> IVGGTASVRGEWPWQVTLHTTSPTQRHLCGGSIIGNQWILTAAHCFYGVESPKILRVYSGILNQSEIKEDTSFFGVQEIIIHDQYKMAESGYDIALLKLETTVGYGDSQRPICLPSKGDRNVIYTDCWVTGWGYRKLRDKIQNTLQKAKIPLVTNEECQKRYRGHKITHKMICA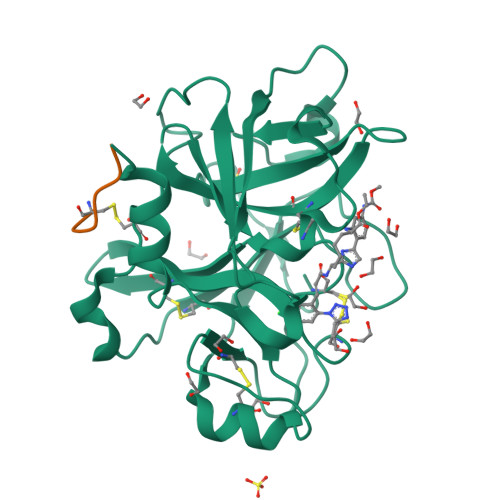GYREGGKDACKGDSGGPLSCKHNEVWHLVGITSWGEGCAQRERPGVYTNVVEYVDWILEKTQAVHHHHHH;> MDDDDKMDNECTTKIKPR> KNPKSDKFK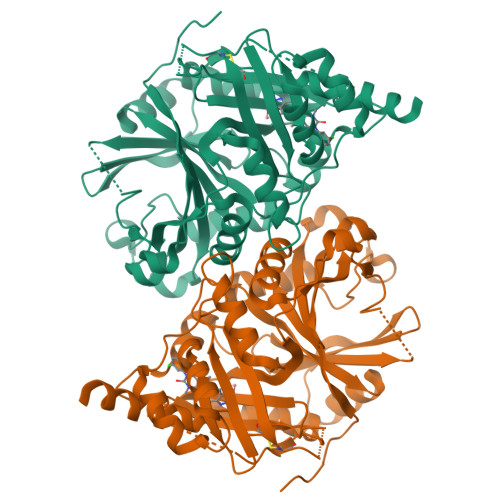VKRFHHIEFWCGDATNVARRFSWGLGMRFSAKSDLSTGNMVHASYLLTSGDLRFLFTAPYSPSLSAGEIKPTTTASIPSFDHGSCRSFFSSHGLGVRAVAIEVEDAESAFSISVANGAIPSSPPIVLNEAVTIAEVKLYGDVVLRYVSYKAEDTEKSEFLPGFERVEDASSFPLDYGIRRLDHAVGNVPELGPALTYVAGFTGFHQFAEFTADDVGTAESGLNSAVLASNDEMVLLPINEPVHGTKRKSQIQTYLEHNEGAGLQHLALMSEDIFRTLREMRKRSSIGGFDFMPSPPPTYYQNLKKRVGDVLSDDQIKECEELGILVDRDDQGTLLQIFTKPLGDRPTIFIEIIQRVGCMMKDEEGKAYQSGGCGGFGKGNFSELFKSIEEYEK> MKKLIPILEKIPEVELPVKEITFKEKLKWTGIVLVLYFIMGCIDVYTAGAQIPAIFEFWQTITASRIGTLITLGIGPIVTAGIIMQLLVGSGIIQMDLSIPENRALFQGCQKLLSIIMCFVEAVLFVGAGAFGILTPLLAFLVIIQIAFGSIILIYLDEIVSKYGIGSGIGLFIAAGVSQTIFVGALGPEGYLWKFLNSLIQGVPNIEYIAPIIGTIIVFLMVVYAECMRVEIPLAHGRIKGAVGKYPIKFVYVSNIPVILAAALFANIQLWGLALYRMGIPILGHYEGGRAVDGIAYYLSTPYGLSSVISDPIHAIVYM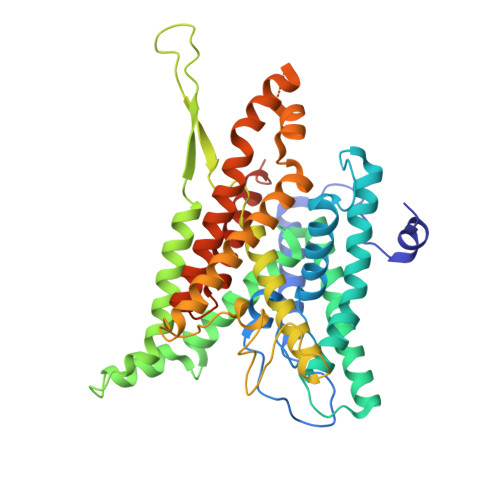IAMIITCVMFGIFWVETTGLDPKSMAKRIGSLGMAIKGFRKSEKAIEHRLKRYIPPLTVMSSAFVGFLATIANFIGALGGGTGVLLTVSIVYRMYEQLLRERTSELHPAIAKLLNK> LPTAQEVQGLMARYIELVDVGDIEAIVQMYADDATVEDPFGQPPIHGREQIAAFYRQGLGGGKVRACLTGPVRASHNGCGAMP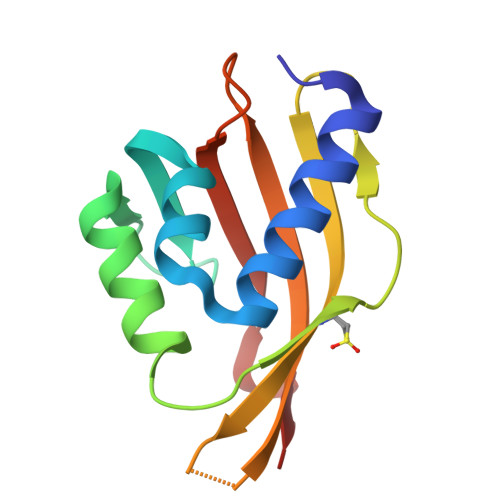FRVEMVWNGQPCALDVIDVARFDEHGRIQTMQAYWSEVNLSV>[2x]GPGSMTVVEAKSRIAVVGGGGSGSVAAWLL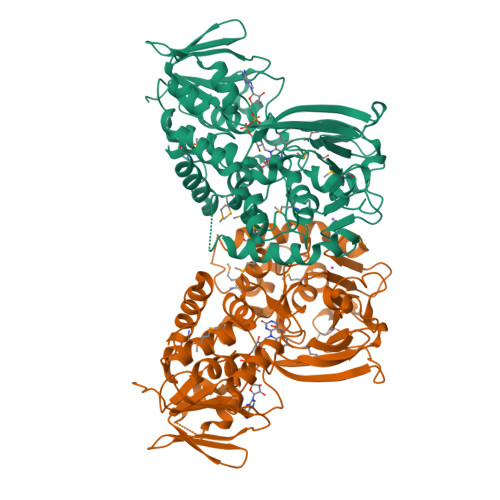ARRHDVTLFEADEYLGGHAYSHPVETDQGTLHVDMGVEHFNEKLSPNLFRLLTDFGIGTYVAPSSVHVDFPGEQQSWNNLDFLGELREELHEEFDRFHQEMNQLPTSGDDSYKQMSIGEYLDKHGYSKSFKYKAMNPILSIYSGCHAPSLDYNLMYVALSFSMNLLSFFSAGYWRKAQGGIHSYLARIESDLGERVRLNTPVEAVVPTQSGVTVLAGGQEHHFDQVVFATHADVTLRLLRTSDQQYRDLLGDFAYVPVESVLHQDESWLSPAGGGAYCQFRMPEGFELARAEEQMGSLTRNCNVLHPYRKVSSPILITFDPQEDVDPERVIVRREWKLPQLRPVDVRRKKRLHEIQGLNGLWFCGTDTSVTGHEGAIVSGMVIADRLGVPHPFPDDAPAAAQFRGIKEFMGV> SNAMGIAARIASAQLQGLVRSRRQVVAGPLVGLLHDEDVWFLSRAVAAEPGVPFDP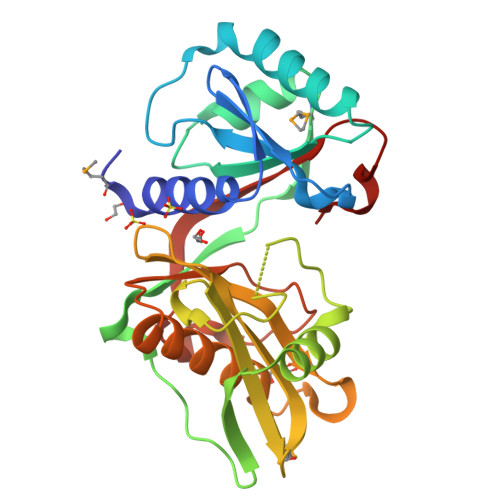AEVPWALETIRKAFAAEDRWLSAELVEEANPGLAYVLVEHGMTIVSRPPLLAVEPGDLLVPEFPAGVTAAVVASAEEQEAANAIAGDAYETDDVASPFQPEPADGGAVLIRMDGVPVATAAWTAIADGVTEVAGVGTLHSHRRQGLGALATAYATQQAFEVGGATLAWLTPGDDGADRIYRRLGYEPKATAVHLGDPGGHLADLR The specific and covalent labeling of the protein HaloTag with fluorescent probes in living cells makes it a powerful tool for bioimaging. However, the irreversible attachment of the probe to HaloTag precludes imaging applications that require transient binding of the probe and comes with the risk of irreversible photobleaching. Here, we introduce exchangeable ligands for fluorescence labeling of HaloTag (xHTLs) that reversibly bind to HaloTag and that can be coupled to rhodamines of different colors. Here, we introduce exchangeable HaloTag Ligands (xHTLs) for the reversible fluorescence labeling of HaloTag7 with rhodamines, opening up new possibilities in bioimaging for a powerful labeling tool.

The binding mode of TMR-S5 and TMR-T5 to HaloTag7 was further studied through X-ray crystallography. The main difference resides in a reorientation of the residues L209 and I211 in order to accommodate the larger trifluoromethyl group in the active site. The L209/I211 conformational change induced by the TMR-T5 binding in the HaloTag7 active site allows a more favorable orientation of the sulfonamide group to form hydrogen bonds with active side residues than observed for TMR-S5; while the TMR-S5 nitrogen-sulfonamide forms a 3.3 Å hydrogen bond with the catalytic D106 carboxylic acid moiety, the corresponding hydrogen bond in bound TMR-T5 is only 2.7 Å. This difference in binding interactions might contribute to the higher affinity of T5-based probes than those of S5-based probes. TMR-linked PEG2-C5-methylsulfonamide (S5) was one of the compounds that presented a lower ΔGbind compared to regular TMR-CA (ΔΔGbind = −4.2 kcal/mol), which displays a KD < 1 μM.6 We synthesized S5 as well as a fluorinated triflamide derivative T5 in order to improve cell permeability and coupled both to fluorogenic rhodamine dyes−34 such as SiR35. The measured kon for these derivatives was above 106 M–1 s–1. Consequently, the koff for the bound probe can be estimated to be around 1 s–1. F/F0 measured for SiR-T5 (12.6 ± 4.0) upon HaloTag7 binding was comparable to the value measured for covalently bound SiR-Halo. The loss of the interaction of the (trifluoromethyl)sulfonamide of xHTLs with D106 resulted in up to 57-fold lower affinities of dHaloTag7 for these probes compared to HaloTag7.

>[2x]GIGTGFPFDPHYVEVLGERMHYVDVGPRDGTPVLFLHGNPTSSYVWRNIIPHVAPTHRCIAPDLIGMGKSDKPDLGYFFDDHVRFMDAFIEALGLEEVVLVIHDWGSALGFHWAKRNPERVKGIAFMEFIRPIPTWDEWPEFARETFQAFRTTDVGRKLIIDQNVFIEGTLPMGVVRPLTEVEMDHYREPFLNPVDREPLWRFPNELPIAGEPANIVALVEEYMDWLHQSPVPKLLFWGTPGVLIPPAEAARLAKSLPNCKAVDIGPGLNLLQEDNPDLIGSEIARWLSTLEI5-chloro-N~4~-cyclopropyl-N~2~-[4-(2-methoxyethoxy)phenyl]pyrimidine-2,4-diamine 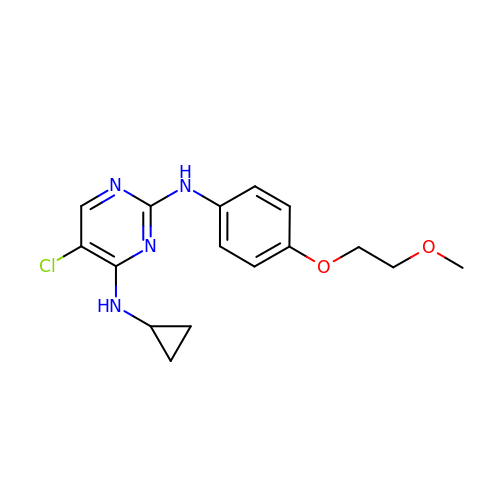| C16 H19 Cl N4 O2 | JFFMERHILPGKFE-UHFFFAOYSA-N> MTFELKRVALPNGIHLDVVDEGPTDAPVLIFLHGFPESHRTWRHQIRHFSDRFRCIAPDQRGYRGSSKPQEVAAYTPDKLIGDIFLLADTLGIGSFTIVGHDWGGAIAW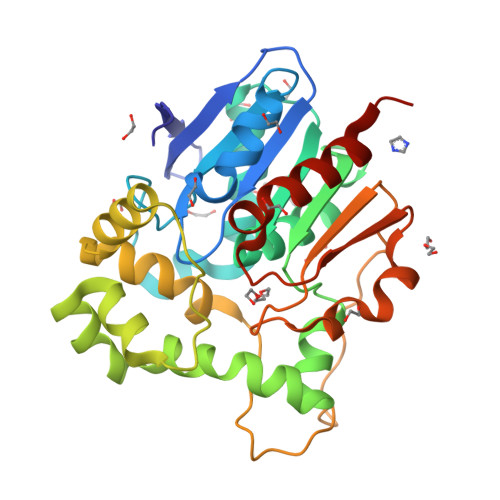GVALGGQHLRVERAIIANAPHPAIFQKLLYTHPVQREASQYIRGFRDPANDALVKEHGLTGLLMKEVKWDRPSAMEPEERDQLLRDWQNHDAAFGMLNYYRASPIDVPTMDAPFKVPAGYTPPQLPRLTIPTLVIWALDDLALPPENLEGLEEIIDPLTIVRVPDCGHFVPWEAPDAVNAAMEGFLAGHHHHHH>GRR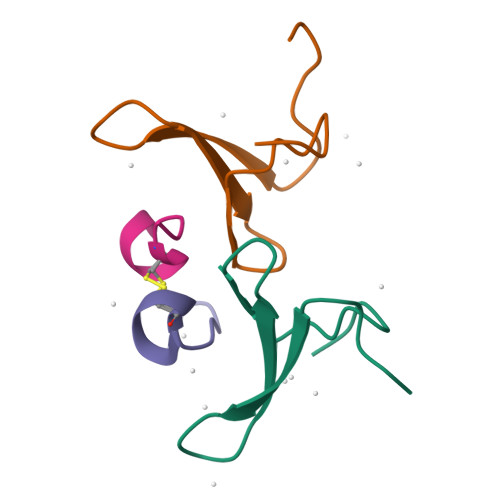ASVELNEKPLPEGWEMRFTVDGIPYFVDHNRRTTTYIDPRTGKS[2x];>XTPEAPPCYMDVIX[2x]>[2x]MAKMRISPELKKLIEKYRCVKDTEGMSPAKVYKL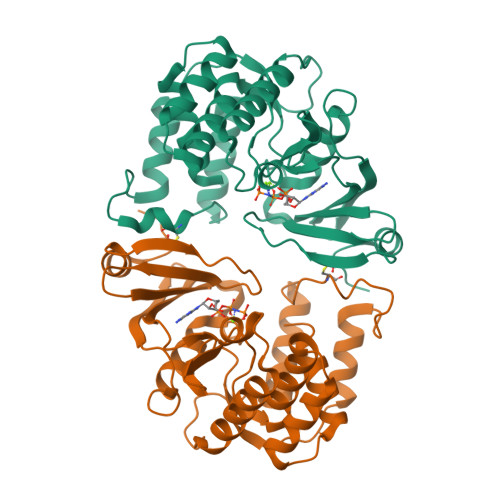VGENENLYLKMTDSRYKGTTYDVEREKDMMLWLEGKLPVPKVLHFERHDGWSNLLMSEADGVLCSEEYEDEQSPEKIIELYAECIRLFHSIDISDCPYTNSLDSRLAELDYLLNNDLADVDCENWEEDTPFKDPRELYDFLKTEKPEEELVFSHGDLGDSNIFVKDGKVSGFIDLGRSGRADKWYDIAFCVRSIREDIGEEQYVELFFDLLGIKPDWEKIKYYILLDELF> MFAWWGRTVYRYRFIVIGVMVALCLGGGVFGLSLGKHVTQSGFYDDGSQSVQASVLGDQVYGRDRSGHIVAIFQAPAGKTVDDPAWSKKVVDELNRFQQDHPDQVLGWAGYLRASQATGMATADKKYTFVSIPLKGDDDDTILNNYKAIAPDLQRLDGGTVKLAGLQPVAEALTGTIATDQRRMEVLALPLVAVVLFFVFGGVIAAGLPVMVGGLCIAGALGIMRFLAIFGPVHYFAQPVVSLIGLGIAIDYGLFIVSRFREEIAEGYDTETAVRRTVITAGRTVTFSAVLIVASAIGLLLFPQGFLKSLTYATIASVMLSAILSITVLPACLGILGKHVDALGVRTLFRVPFLANWKISAAYLNWLADRLQRTKTREEVEAGFWGKLVNRVMKRPVLFAAPIVIIMILLIIPVGKLSLGGISEKYLPPTNSVRQAQEEFDKLFPGYRTNPLTLVIQTSNHQPVTDAQIADIRSKAMAIGGFIEPDNDPANMWQERAYAVGASKDPSVRVLQNGLINPADASKKLTELRAITPPKGITVLVGGTPALELDSIHGLFAKMPLMVVILLTTTIVLMFLAFGSVVLPIKATLMSALTLGSTMGILTWIFVDGHFSKWLNFTPTPLTAPVIGLIIALVFGLSTDYEVFLVSRMVEARERGMSTQEAIRIGTAATGRIITAAALIVAVVAGAFVFSDLVMMKYLAFGLMAALLLDATVVRMFLVPSVMKLLGDDCWWAPRWARRLQTRIGLGEIHLPDGSENLYFQ

MmpL3 is an essential protein belonging to the resistance-nodulation-division (RND) superfamily of transporters (DeJesus et al., 2017; Domenech et al., 2005). Specifically, MmpL3 exports intracellularly synthesized trehalose monomycolate (TMM) into the periplasm (Grzegorzewicz et al., 2012). TMM transport is essential for the formation of the unique Mycobacterium cell envelope that functions as the main physical barrier to drug entry and neutralization by the immune system (Dulberger et al., 2020; Jackson, 2014). The driving force for TMM export is thought to come from the proton-motive force (PMF) established across the inner membrane (Grzegorzewicz et al., 2012; Székely and Cole, 2016), although the precise mechanism by which the PMF drives lipid export remains unclear.

To obtain the structure of Mtb MmpL3 we generated a C-terminally truncated (residues 1–753) construct capable of being overexpressed in E. coli. However, cryo-EM imaging of the protein purified in lauryl maltose neopentyl glycol (LMNG) permitted its three-dimensional reconstruction to a resolution of 3.0 Å. Our map reveals MmpL31-753 to be monomeric, consistent with the Msmg homolog (Su et al., 2019; Zhang et al., 2019). Mtb MmpL31-753 adopts a transmembrane domain (TMD) fold archetypal of RND proteins, consisting of 12 transmembrane helices (TMs) arranged as two sequence-contiguous bundles (TMs 1–6 and 7–12). Characteristic of RND transporters, sizable periplasmic loops connect TMs 1–2 in the N-terminal half of MmpL31-753 (PN, residues 37–166) and TMs 7–8 (PC, residues 415–544) in the C-terminal half of the molecule. Similar to structures of the Msmg MmpL3 homolog (Su et al., 2019; Zhang et al., 2019), the Mtb protein has an extensive cavity enclosed by the PD. Within this cavity a lipid-like species was captured in our structure, most likely the detergent LMNG, which adopts a splayed arrangement bound between the PN and PC subdomains. LMNG creates a substantial interface, packing against 35 residues (within 4.5 Å) and sitting within the suggested transport path for TMM (Klenotic et al., 2020). Structural comparison with the Mtb MmpL31-753-LMNG complex identifies striking similarities in the binding poses of all four ligands.>[4x]MQIRDWLPLLGMPLMLLFVQIIAIVLVMPMQAAGLVAFENPSSVANPLIFIGMLLAFTLVLLVLLRTGGRRFIAAFIGFALFMTFLYIFGALSLLALGPTTAAAAGTLIGAVAVTALLYLYPEWYVIDILGVLISAGVASIFGISLEPLPVLVLLVLLAVYDAISVYRTKHMITLAEGVLETKAPIMVVVPKRADYSFRKEGLNISEGEERGAFVMGMGDLIMPSILVVSSHVFVD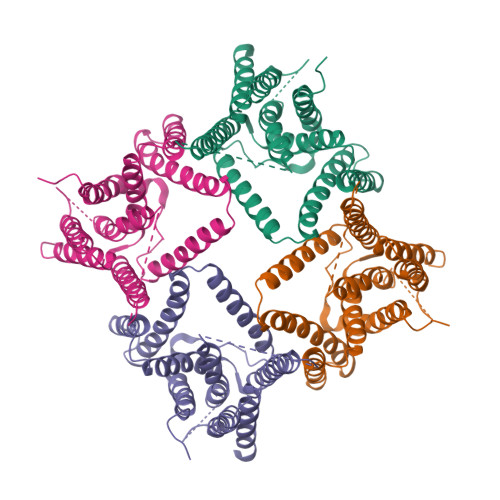APAVLWTLSAPTLGAMVGSLVGLAVLLYFVNKGNPQAGLPPLNGGAILGFLVGAALAGSFSWLPF>MSQHNEKNPHQHQSPLHDSSEAKPGMDSLAPEDGSHRPAAEPTPPGAQPTAPGSLKAPDTRNEKLNSLEDVRKGSENYALTTNQGVRIADDQNSLRAGSRGPTLLEDFILREKITHFDHERIPERIVHARGSAAHGYFQPYKSLSDITKADFLSDPNKITPVFVRFSTVQGGAGSADTVRDIRGFATKFYTEEGIFDLVGNNTPIFFIQDAHKFPDFVHAVKPEPHWAIPQGQSAHDTFWDYVSLQPETLHNVMWAMSDRGIPRSYRTMEGFGCHTFRLINAEGKATFVRFHWKPLAGKASLVWDEAQKLTGRDPDFHRRELWEAIEAGDFPEYELGFQLIPEEDEFKFDFDLLDPTKLIPEELVPVQRVGKMVLNRNPDNFFAENEQAAFHPGHIVPGLDFTNDPLLQGRLFSYTDTQISRLGGPNFHEIPINRPTAPYHNFQRDGMHRMGIDTNPANYEPNSINDNWPRETPPGPKRGGFESYQERVEGNKVRERSPSFGEYYSHPRLFWLSQTPFEQRHIVDGFSFELSKVV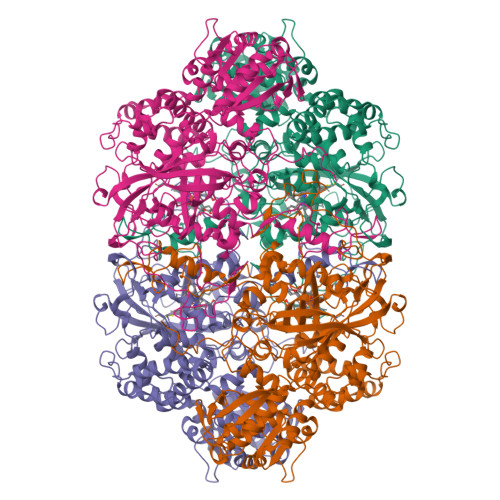RPYIRERVVDQLAHIDLTLAQAVAKNLGIELTDDQLNITPPPDVNGLKKDPSLSLYAIPDGDVKGRVVAILLNDEVRSADLLAILKALKAKGVHAKLLYSRMGEVTADDGTVLPIAATFAGAPSLTVDAVIVPAGNIADIADNGDANYYLMEAYKHLKPIALAGDARKFKATIKIADQGEEGIVEADSADGSFMDELLTLMAAHRVWSRIPKIDKIPA[4x]> AIRNCIIGKGRSYKGTVSITKSGIKCQPWSSMIPHEHSFLPSSYRGKDLQENYCRNPRGEEGGPWCFTSNPEVRYEVCDIPQCSEVECIIGKGRSYKGTVSITKSGIKCQPWSSMIPHEHSFLPSSYRGKDLQENYCRNPRGEEGGPWCFTSNPEVRYEVCDIPQCSEVEHHHHHH

In this work, we describe the rational design, production, and characterization of K1K1, a novel minimal MET agonist consisting of two copies of the kringle 1 domain of HGF/SF in tandem orientation. On the strength of the structural, biochemical, and mutagenesis data available, we rationalized that a covalent dimer containing a tandem repeat of the K1 domain of HGF/SF could constitute a minimal and stable MET agonist able to diffuse effectively across tissue boundaries owing to the absence of the N-terminal domain of HGF/SF responsible for high-affinity binding to heparan sulphate proteoglycans (HSPG). Therefore, we designed a linker to bridge the distance between the C-terminus of the first K1 domain and the N-terminus of the second one. We chose for that purpose the four–amino acid long linker, SEVE, which is naturally present between kringle 1 and kringle 2 (K2) in HGF/SF.

Furthermore, a poly-histidine–tagged variant, designated K1K1H6, was produced to facilitate certain assays and a single kringle 1 domain poly-histidine–tagged variant (K1H6) as a monovalent control. The collected datasets enabled the determination of the molecular structures at 1.8 Å resolution and 1.7 Å for K1K1 and K1K1H6, respectively. Both proteins crystalized in space group P 1 21 1 with K1K1 having two molecules per asymmetric unit and K1K1H6 having one. Structurally, K1K1 and K1K1H6 are nearly identical with a backbone root mean square deviation of 0.8 or 1.8 Å, depending on which of the two molecules in the asymmetric unit of K1K1 is used for alignment with K1K1H6. Both proteins show an elongated “stretched-out” conformation with the MET-binding sites exposed on opposite ends and the N- and C-terminus located at the centre. In K1K1H6, good electron density was also observed for the poly-histidine tag possibly because of stabilising interactions between the histidine residues and residues of the N-terminal kringle domain. The C-terminal poly-histidine tag of K1K1H6 is making contacts with residues in the N-terminal kringle domain. Surprisingly, like the revelation of seeing the first structures of NK1 that presented a likely biologically relevant dimer, both crystal structures show a pseudo C2 symmetry around a central axis and present both receptor-binding sites in nearly identical orientation on either side of the molecule (located around residue Glu37 in the first kringle and residues Glu120 in the second kringle, equivalent to NK1 residue Glu159). For p-Akt, both K1K1H6 and K1K1 show similar phosphorylation in the low nanomolar range with no significant effect caused by the presence or absence of the poly-histidine tag. We next confirmed the direct binding of K1K1H6 to recombinant human MET-Fc chimera, a soluble dimeric protein comprising the whole extracellular part of the MET receptor (MET922 fused to the Fc region of human IgG1) at different concentrations using the AlphaScreen technology.>[5x]MKIFLDTAN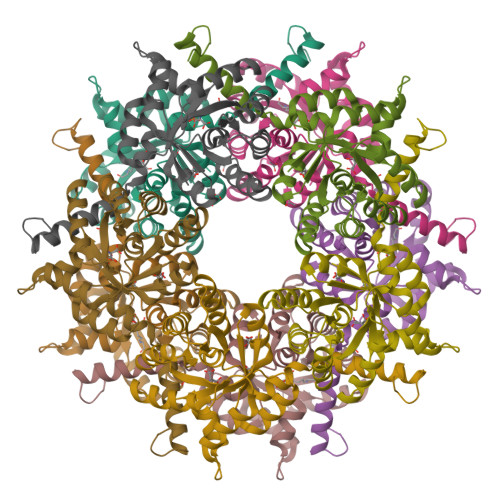IDEIRTGVNWGIVDGVTTNPTLISKEAVNGKKYGDIIREILKIVDGPVSVEVVSTKYEGMVEEARKIHGLGDNAVVKIPMTEDGLRAIKTLSSEHINTNCTLVFNPIQALLAAKAGVTYVSPFVGRLDDIGEDGMQIIDMIRTIFNNYIIKTQILVASIRNPIHVLRSAVIGADVVTVPFNVLKSLMKHPKTDEGLAKFLEDWKKVSPDGKLIL> CCGGACGAGGUGCGCCGUACCCGGUCAGGACAAGACGGCGC;> CCGGACGAGGUGCGCCGUACCCGGUCACGACAAGACGGCGC

We have determined high-resolution crystal structures of the ykkC guanidine III riboswitch from Thermobifida fusca. X-ray crystallography shows that the RNA folds into an H-type pseudoknot, in which a connecting strand locates in the major groove of one duplex to form a regular triple helix. This continues into the central core of conserved nucleotides that form a novel left-handed helical ramp of inter-nucleotide interactions, generating the guanidinium cation binding site. Comparison with earlier probing data suggest that the formation of the triple helix is stabilized by guanidine binding and this exposes the adjacent ribosome binding site to permit initiation of gene translation.

Methylguanidine and aminoguanidine were co-crystallized with the riboswitch RNA, while ethylguanidine and agmatine were soaked into ligand-free crystals. All crystallized in the trigonal space group P3121, and all diffracted to good resolution (2.01–2.32 Å). However, the side opening cannot readily accommodate longer alkyl chains, and agmatine was bound in a significantly different manner. The ligand was found to be rotated by 120° in the binding pocket so that the butylamine side chain is attached to the guanidine nitrogen that is hydrogen bonded to G7 N7, and consequently there is no hydrogen bond to C6 O2'. The trajectory of the butylamine side chain is quite different from those of the other ligands, being directed upwards along the groove in the RNA structure. We also show that agmatine may bind to the guanidine III riboswitch, but in a different manner that involves a rotation of the guanidino nucleus. The side opening can accommodate a range of small side chains, with affinities in the order guanidine > methylguanidine ∼ aminoguanidine > ethylguanidine > agmatine. In principle arginine might be accommodated in the same manner as agmatine, but it is likely that the additional carboxylate group of the amino acid adds further destabilization leading to an unmeasurable affinity.>SMGRDAPAPAASQPSGCGKHNSPERKVYMDYNATTPLEPEVIQAMTKAMWEAWGNPSSPYSAGRKAKDIINAARESLAKMIGGKPQDIIFTSGGTESNNLVIHSVVKHFHANQTSKGHTGGHHSPVKGAKPHFITSSVEHDSIRLPLEHLVEEQVAAVTFVPVSKVSGQTEVDDILAAVRPTTRLVTIMLANNETGIVMPVPEISQRIKALNQERVAAGLPPILVHTDAAQALGKQRVDVEDLGVDFLTIVGHKFYGPRIGALYIRGLGEFTPLYPMLFGGGQERNFRPGTENTPMIAGLGKAAELVTQNCEAYEAHMRDVRDYLEERLEAEFGQKRIHLNSQFPGTQRLPNTCNFSIRGPRLQGHVVLAQCRVLMASVGAACHSDHGDQPSPVLLSYGVPFDVARNAL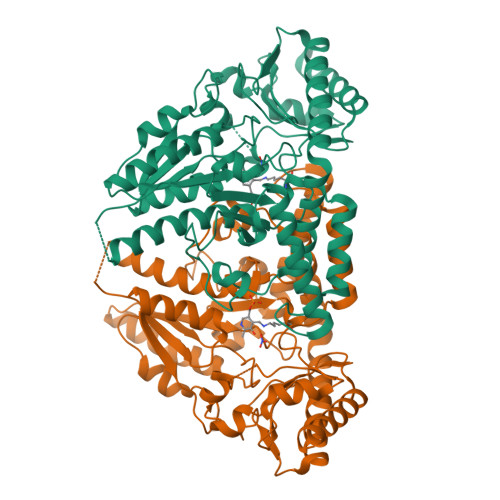RLSVGRSTTRAEVDLVVQDLKQAVAQLEDQA[4x]> MSMLKREDWYDLTRTTNWTPKYVTENELFPEEMSGARGISMEAWEKYDEPYKITYPEYVSIQREKDSGAYSIKAALERDGFVDRADPGWVSTMQLHFGAIALEEYAASTAEARMARFAKAPGNRNMATFGMMDENRHGQIQLYFPYANVKRSRKWDWAHKAIHTNEWAAIAARSFFDDMMMTRDSVAVSIMLTFAFETGFVNMQFLGLAADAAEAGDHTFASLISSIQTDESRHAQQGGPSLKILVENGKKDEAQQMVDVAIWRSWKLFSVLTGPIMDYYTPLESRNQSFKEFMLEWIVAQFERQLLDLGLDKPWYWDQFMQ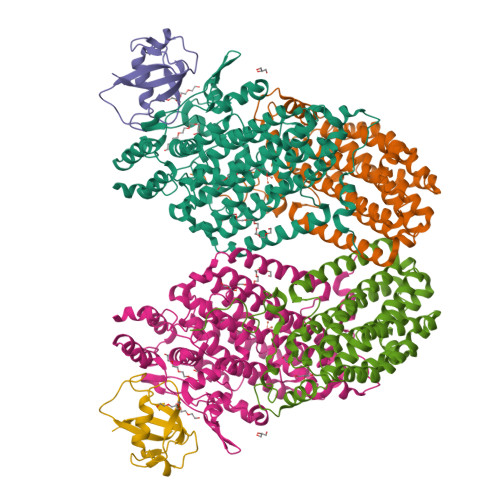DLDETHHGMHLGVWYWRPTVWWDPAAGVSPEEREWLEEKYPGWNDTWGQCWDVITDNLVNGKPELTVPETLPTICNMCNLPIAHTPGNKWNVKDYQLEYEGRLYHFGSEADRWCFQIDPERYENHTNLVDRFLKGEIQPADLAGALMYMSLEPGVMGDDAHDYEWVKAYQKKTNAA;> MSEQQPEALKPLKTWSHLAGNRRRPSEYEVVSTNLHYFTDNPERPWELDSNLPMQTWYKKYCFDSPLKHDDWNAFRDPDQLVYRTYNLLQDGQESYVQGLFDQLNDRGHDQMLTREWVETLARFYTPARYLFHALQMGSVYIHQIAPASTITNCATYETADHLRWLTHTAYRTRELANCYPDVGFGKRERDVWENDPAWQGFRELIEKALIAWDWGEAFTAINLVTKPAVEEALLQQLGSLAQSEGDTLLGLLAQAQKRDAERHRRWSSALVKMALEKEGNREVLQKWVAKWEPLADKAIEAYCSALPDGENAIVEAKSASRYVRQMMGL;> MATFPIMSNFERDFVIQLVPVDTEDTMDQVAEKCAYHSINRRVHPQPEKILRVRRHEDGTLFPRGMIVSDAGLRPTETLDIIFMDN> GAMGEELTLTILRQTGGLGISIAGGKGSTPYKGDDEGIFISRVSEEGPAARAGVRV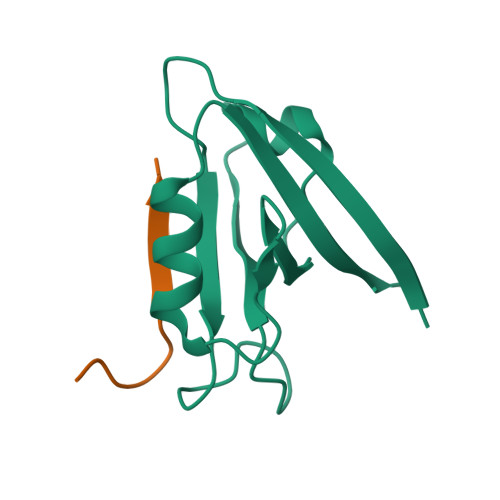GDKLLEVNGVALQGAEHHEAVEALRGAGTAVQMRVWRER;> XKPNGLLITDFPX> GSHHHHHHSQDPMPTPLPQLPSNVRDGENNVASTFLQAFFQLWDHDRLTLIPQFYDSETTFSVVFATDSPQDPASSSCSKFSRNLNILSPRHPSTLQRLFVGSNLIADLWKVLPATRHPSLDQTSQWLIDCHTFPHLADPTGMAPYAMGLMINVNGQCEEADISQNLYGTRTFSRCFILGPSKPGAPHPYRVLSDQLTLHTWKPQPAPQVGTV;> MLSRRYAAKSFVEWYYRQINENKPVASGYVNNNATYTKAGHPP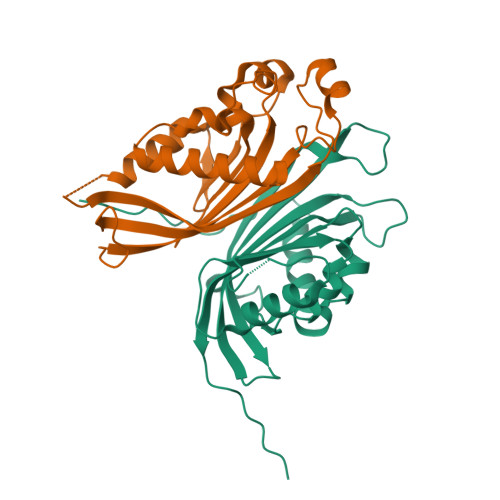ADITINGRVVATPEEWDTMLKEQRAQHNTSSSSTLPIGRKPVRYDVDCFDVHVINADYRFAAPQRMIEQHAPTDGVRMMMALTVSGSVYFGASPRSTDDYVIKQHFNDVFILVPNWDVLEKPGARSARKYLIASHKYRAY The bacterial flagellar motor is a huge bidirectional rotary nanomachine that drives rotation of the flagellum for bacterial motility. The cytoplasmic C ring of the flagellar motor functions as the switch complex for the rotational direction switching from counterclockwise to clockwise. The basal body is made up of the LP ring, MS ring, C ring, rod and export apparatus. Here, we present two high-resolution cryo-electron microscopy structures of the C ring-containing flagellar basal body–hook complex from Salmonella Typhimurium, which are in the default counterclockwise state and in a constitutively active CheY mutant-induced clockwise state, respectively.

2D classification results showed that the C ring in the CW state (CW-C ring) also possesses a C34 symmetry. The density map of the C ring in the CW state was finally refined to an overall resolution of 5.6 Å with C34 symmetry. The subunits of CheY** and the CW-C ring have clear densities in the density map. There are in all 34 CheY** subunits, which are bound on the outer surface of the middle subring of the C ring and form a CheY** subring structure. The CheY**-bound C ring in the CW state has a height of ~160 Å, which is the same as that of the C ring in the CCW state. However, the upper, middle and bottom subrings of the CW-C ring have diameters of ~446 Å, ~440 Å and ~470 Å, respectively, which are all smaller than those in the CCW-C ring, indicating that the binding of CheY** induces a more compressed structure of the C ring. The inner diameter of the inner subring is also shortened to ~312 Å. CheY** is bound into an open groove between two adjacent protomers on the surface of the middle subring of the C ring and interacts with FliGM, FliMM and the prior FliMM domain. However, in contrast to previous predictions, CheY** has no interactions with FliN and the bottom subring in the structure. As the consequence, the whole FliGCC domain undergoes a rotation by ~180° and a movement by ~8 Å toward the next FliGCC domain and inward contraction by ~10 Å to the center of the C ring, which results in a reversed orientation of the αtorque helix and changes the periodic CCW distribution of the charged residues R281 and D288/D289 to a CW distribution on the upper surface of the CW-C ring.

>[102x]MSDMNNPSDENTGALDDLWADALNEQKATTTKSAADAVFQQLGGGDVSGAMQDIDLIMDIPVKLTVELGRTRMTIKELLRLTQGSVVALDGLAGEPLDILINGYLIAQGEVVVVADKYGVRITDIITPSERMRRLSR;>[34x]MSNLSGTDKSVILLMTIGEDRAAEVFKHLSTREVQALSTAMANVRQISNKQLTDVLSEFEQEAEQFAALNINANEYLRSVLVKALGEERASSLLEDILETRDTTSGIETLNFMEPQSAADLIRDEHPQIIATILVHLKRSQAADILALFDERLRHDVMLRIATFGGVQPAALAELTEVLNGLLDGQNLKRSKMGGVRTAAEIINLMKTQQEEAVITAVREFDGELAQKIIDEMFLFENLVDVDDRSIQRLLQEVDSESLLIALKGAEPPLREKFLRNMSQRAADILRDDLANRGPVRLSQVENEQKAILLIVRRLAETGEMVIGSGEDTYV;>MADKELKFLVVDKFSTMRRIVRNLLKELGFNNVEEAEDGVDALNKLQAGGFGFIISDWNMPNMDGLELLKTIRADSAMSALPVLMVTAEAKKENIIAAAQAGASGWVVKPFTAATLEEKLNKIFEKLGM[34x];>MGDSILSQAEIDALLNGDSDTKDEPTPGIASDSDIRPYDPNTQRRVVRERLQALEIINERFARQFRMGLFNLLRRSPDITVGAIRIQPYHEFARNLPVPTNLNLIHLKPLRGTGLVVFSPSLVFIAVDNLFGGDGRFPTKVEGREFTHTEQRVINRMLKLALEGYSDAWKAINPLEVEYVRSEMQVKFTNITTSPNDIVVNTPFHVEIGNLTGEFNICLPFSMIEPLRELLVNPPLENSRHEDQNWRDNLVRQVQHSELELVANFADIPLRLSQILKLKPGDVLPIEKPDRIIAHVDGVPVLTSQYGTVNGQYALRVEHLINPILNSLNEEQPK[34x];>MSATASTATQPKPLEWLNRLRANPRIPLIVAGSAAVAIVVAMVLWAKTPDYRTLFSNLSDQDGGAIVAQLTQMNIPYRFANGSGAIEVPADKVHELRLRLAQQGLPKGGAVGFELLDQEKFGISQFSEQVNYQRALEGELARTIETLGPVKSARVHLAMPKPSLFVREQKSPSASVTVTLEPGRALDEGQISAVVHLVSSAVAGLPPGNVTLVDQSGHLLTQSNTSGRDLNDAQLKFANDVESRIQRRIEAILSPIVGNGNVHAQVTAQLDFANKEQTEEHYSPNGDASKATLRSRQLNISEQVGAGYPGGVPGALSNQPAPPNEAPIATPPTNQQNAQNTPQTSTSTNSNSAGPRSTQRNETSNYEVDRTIRHTKMNVGDIERLSVAVVVNYKTLADGKPLPLTADQMKQIEDLTREAMGFSDKRGDTLNVVNSPFSAVDNTGGELPFWQQQSFIDQLLAAGRWLLVLVVAWILWRKAVRPQLTRRVEEAKAAQEQAQVRQETEEAVEVRLSKDEQLQQRRANQRLGAEVMSQRIREMSDNDPRVVALVIRQWMSNDHE[34x]1-acetyl-4-(4-{[(2R,4S)-2-(2,4-dichlorophenyl)-2-(1H-imidazol-1-ylmethyl)-1,3-dioxolan-4-yl]methoxy}phenyl)piperazine | C26 H28 Cl2 N4 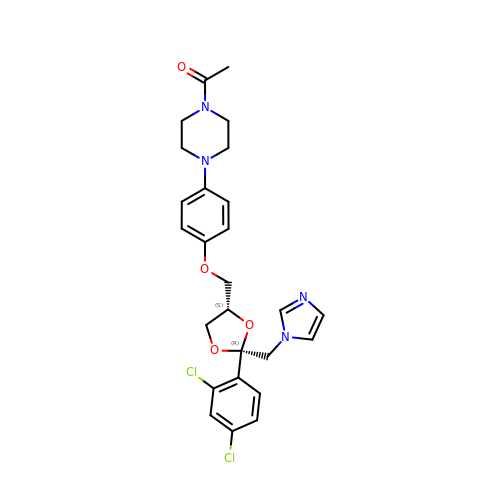O4 | XMAYWYJOQHXEEK-OZXSUGGESA-N> MARGLNRVFLIGALATRPDMRYTPAGLAILDLTLAGQDLLLSDNGGEREVSWYHRVRLLGRQAEMWGDLLDQGQLVFVEGRLEYRQWEREGERRSELQIRADFLDPLDDRGKERAEDSRGQPRLRAALNQVFLMGNLTRDPELRYTPQGTAVARLGLAVNERRQGAEERT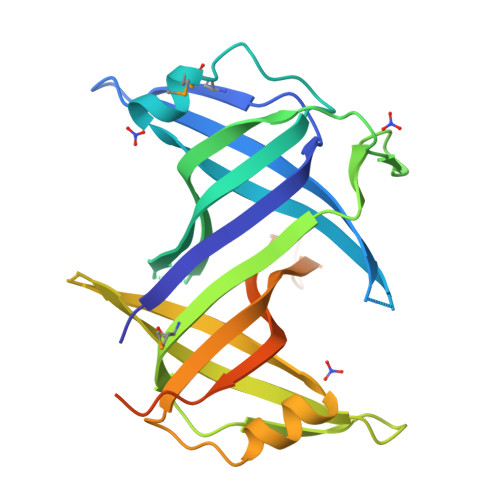HFVEVQAWRDLAEWAAELRKGDGLFVIGRLVNDSWTSSSGERRFQTRVEALRLERPTRGPAQAGGSRSREVQTGGVDIDEGLEDFPPEEELPF2-[(9H-carbazol-3-yl)oxy]-N,N-dimethylethan-1-amine | C16 H18 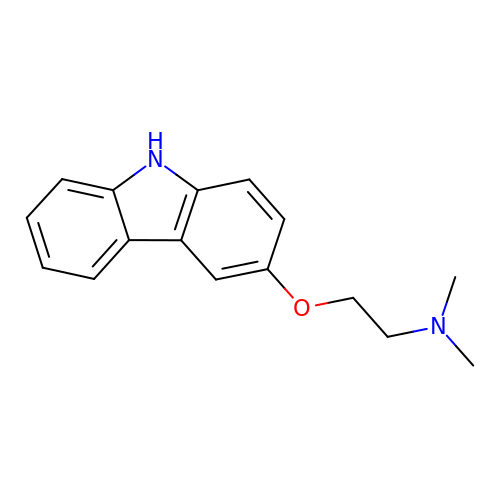N2 O | IIXIJWXGDDCXBA-UHFFFAOYSA-N> MGHHHHHHHMEFGSMPATRKPMRYGHTEGHTEVCFDDSGSFIVTCGSDGDVRIWEDLDDDDPKFINVGEKAYSCALKSGKLVTAVSNNTIQVHTFPEGVPDGILTRFTTNANHVVFNGDGTKIAAGSSDFLVKIVDVMDSSQQKTFRGHDAPVLSLSFDPKDIFLASASCDGSVRVWQISDQTCAISWPLLQKCNDVINAKSICRLAWQPKSG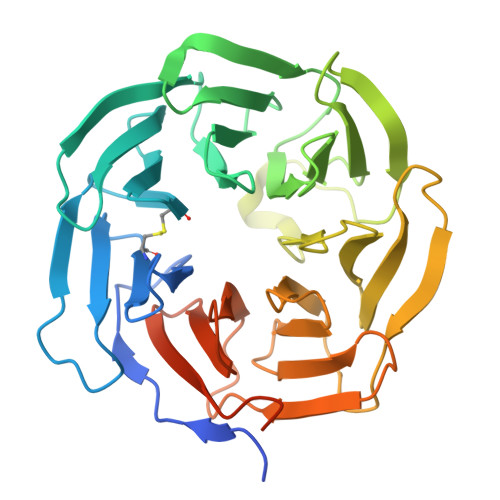KLLAIPVEKSVKLYRRESWSHQFDLSDNFISQTLNIVTWSPCGQYLAAGSINGLIIVWNVETKDCMERVKHEKGYAICGLAWHPTCGRISYTDAEGNLGLLENVCDPSGKTSSSKVSSRVEKDYNDLFDGD>SQANLMRLKSDLFNRSPMYPGPTKDDPLTVTLGFTLQDIVKVDSSTNEVDLVYYEQQRWKLNSLMWDPNEYGNITDFRTSAADIWTPDITAYSSTRPVQVLSPQIAVVTHDGSVMFIPAQRLSFMCDPTGVDSEEGVTCAVKFGSWVYSGFEIDLKTDTDQVDLSSYYASSKYEILSATQTRQVQHYSCCPEPYIDVNLVVKFRER[6x];>QANLMRLKSDLFNRSPMYPGPTKDDPLTVTL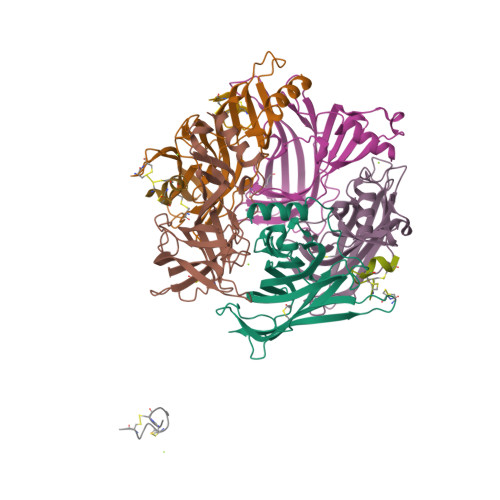GFTLQDIVKVDSSTNEVDLVYYEQQRWKLNSLMWDPNEYGNITDFRTSAADIWTPDITAYSSTRPVQVLSPQIAVVTHDGSVMFIPAQRLSFMCDPTGVDSEEGVTCAVKFGSWVYSGFEIDLKTDTDQVDLSSYYASSKYEILSATQTRQVQHYSCCPEPYIDVNLVVKFRE[2x];>SQANLMRLKSDLFNRSPMYPGPTKDDPLTVTLGFTLQDIVKVDSSTNEVDLVYYEQQRWKLNSLMWDPNEYGNITDFRTSAADIWTPDITAYSSTRPVQVLSPQIAVVTHDGSVMFIPAQRLSFMCDPTGVDSEEGVTCAVKFGSWVYSGFEIDLKTDTDQVDLSSYYASSKYEILSATQTRQVQHYSCCPEPYIDVNLVVKFRE[2x];>[8x]GCCSDPRCRYRCR> MAELACFCYPHLENDSYKFIPFNNLAIKAMLTAKVDKKDMDKFYDSIIYGIAPPPQFKKRYNTNDNSRGMNFETIMFTKVAMLICEALNSLKVTQANVSNVLSRVVSIRHLENLVIRKENPQDILFHSKDLLLKSTLIAIGQSKEIETTITAEGGEIVFQNAAFTMWKLTYLEHQLMPILDQNFIEYKVTLNEDKPISDVHVKELVAELRWQYNKFAVITHGKGHYRIVKYSSVANHADRVYATFKSNVKTGVNNDFNLLDQR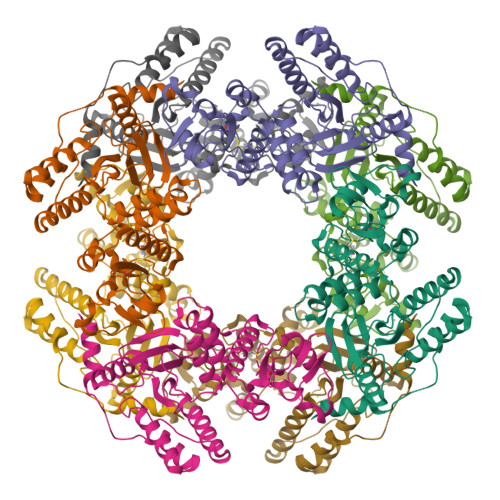IIWQNWYAFTSSMKQGNTLDVCKRLLFQKMKPEKNPFKGLSTDRKMDEVSQVGVLVPR>MGQLYIVPTPIGNLADITQRALEVLQAVDLIAAEDTRHTGLLLQHFGINARLFALHDHNEQQKAETLLAKLQEGQNIAL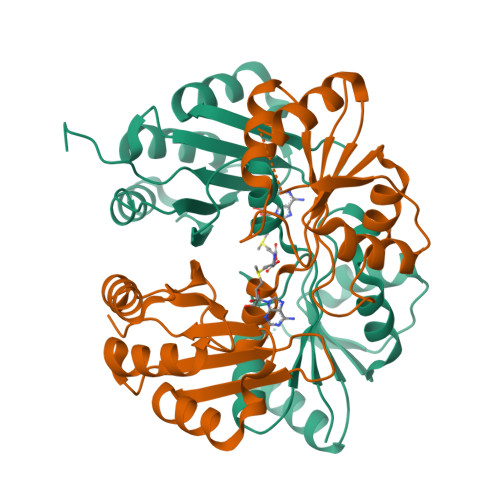VSDAGTPLINDPGYHLVRTCREAGIRVVPLPGPCAAITALSAAGLPSDRFCYEGFLPAKSKGRRDALKAIEAEPRTLIFYESTHRLLDSLEDIVAVLGESRYVVLARELTKTWETIHGAPVGELLAWVKEDENRRKGEMVLIVEGHKAQEEDLPADALRTLALLQAELP[3x]> NGNYDYLMYADIDYDHPDVAAEIKRWGTWYANELQLDGFRLDAVKHIKFSFLRDWVNHVREKTGKEMFTVAEYWQNDLGALENYLNKTNFNHSVFDVPLHYQFHAASTQGGGYDMRKLLNSTVVSKHPLKAVTFVDNHDTQPGQSLESTVQTWFKPLAYAFILTRESGYPQVFYGDMYGTKGDSQREIPALKHKIEPILKARKQYAYGAQHDYFDHHDIVGWTREGDSSVANSGLAALITDGPGGAKRMYVGRQNAGETWHDITGNRSEPVVINS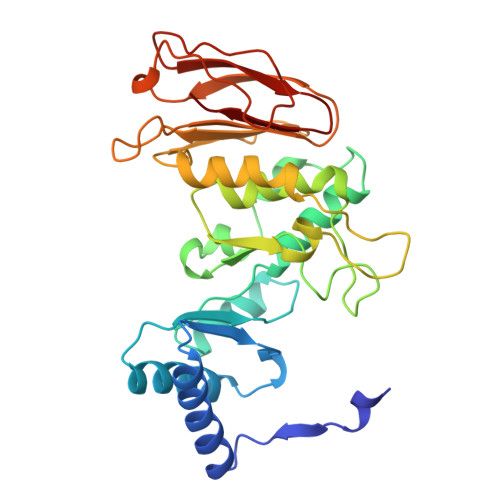EGWGEFHVNGGSVSIYVQR> GSHHVVPNEVVVQRLFQVKGRRVVRATEVPVSWESFNNGDCFILDLGNNIHQWCGSNSNRYERLKATQVSKGIRDNE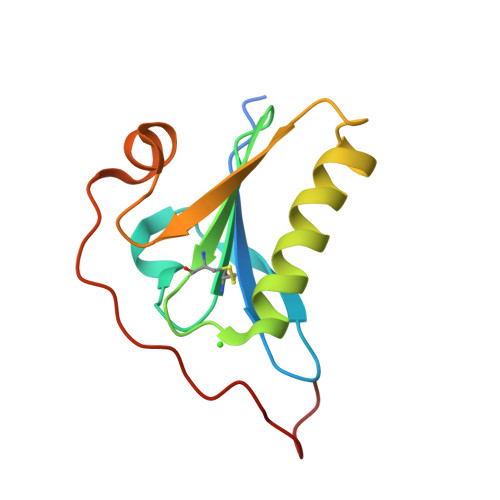RSGRARVHVSEEGTEPEAMLQVLGPKPALPAGTEDTAKEDAA> GPLGSHMGARNGRAGPSDSAFSFTKSRARVLTEAPKVTFKDVAGAEEAKEELKEIVEFLKNPSRFHEMGARIPKGVLLVGPPGVGKTHLARAVAGEARVPFITASGSDFVEMFVGVG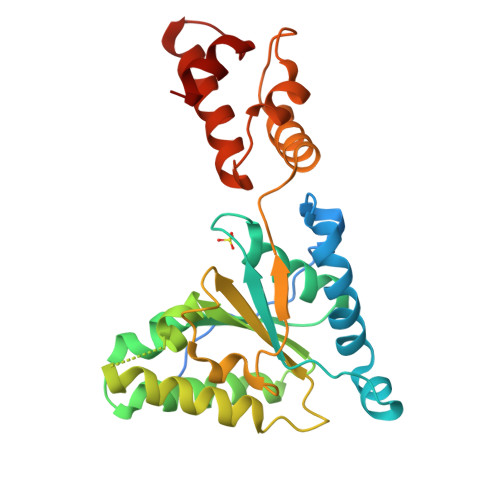AARVRDLFETAKRHAPCIVFIDEIDAVGRKRGSGVGGGNDEREQTLNQLLVEMDGFEKDTAIVVMAATNRPDILDPALLRPGRFDRQIAIDAPDVKGREQILRIHARGKPLAEDVDLALLAKRTPGFVGADLENLLNEAALLAAREGRRKITMKDLEEAAS> GPGMAPVPTGVFTDIPISNIRRVIAQRLMQSKQTIPHYYLSIDVNMGEVLLVRKELNKILEGRSKISVNDFI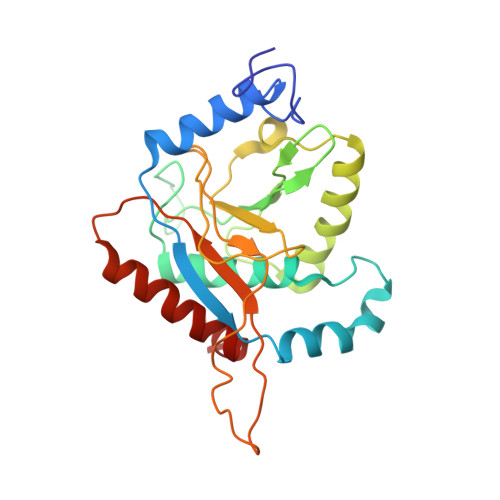IKASALACLKVPEANSSWMDTVIRQNHVVDVSVAVSTPAGLITPIVFNAHIKGVETIANDVVSLATKAREGKLQPHEFQGGTFTISNLGMFGIKNFSAIINPPQACILAIGASEDKLVPADNEKGFDVASMMSVTLSCDHRVVDGAVGAQWLAEFRKYLEKPITMLL>[8x]MTNTVSTMILFGSTGDLSQRMLLPSLYGLDADGLLADDLRI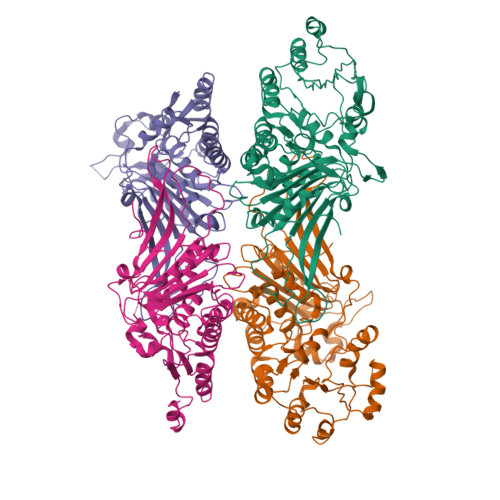VCTSRSEYDTDGFRDFAEKALDRFVASDRLNDDAKAKFLNKLFYATVDITDPTQFGKIADLCGPVEKGIAIYLSTSPSLFEGAIAGLKQAGLAGPTSRLALEKPLGQDLASSDHINDAVLKVFSEKQVYRIDHYLGKETVQNLLTLRFGNALFEPLWNSKGIDHVQISVAETVGLEGRIGYFDSSGSLRDMVQSHILQLVALVAMEPPAHMEANAVRDEKVKVFRALRPINNDTVITHTVTGQYGAGVSGGKEVAGYIDELGQPSDTETFVAIKAHVDNWRWHGVPFYIRTGKRLPARRSEIVVQFKPVPHSIFSSSGGILQPNKLRIVLQPDETIQISIMVKEPGLDRNGAHMREVWLDLSLTDVFKDRKRRIAYERLMLDLIEGDATLFVRRDEVEAQWIWIDGIREGWKANSMKPKTYVSGTWGPITAIALVERDGVTWYDLEHHHHHH> SRRVASPSSELRRALEANEFIPYYQPLSPGQGGRWIGVEVLMRWRHPREGLIRPDLFIPFAERSGLIVPMTRALMRQVAEDLGGHAGKLEPGFHIGFNISATHCHELALVDDCRELLAAFPPGHITLVLELTERELIESSEVTDRLFDELHALGVKIAIDDFGTGHSSLAYLRKFQVDCLKIDQSFVARIGIDTLSGHILD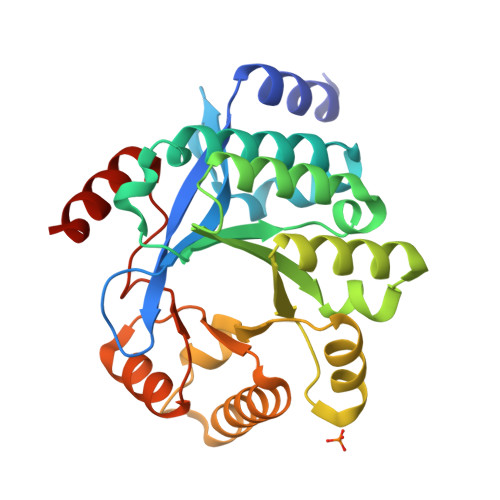SIVELSAKLDLDIVAEGVETPEQRDYLAARGVDYLQGYLIGRPMPLESLLSSLTVQEQQGAS>[2x]DYKDDDDKHHHHHHHHHHLEVLFQGPQSSERRVVAHMPGDIIIGALFSVHHQPTVDKVHERKCGAVREQYGIQRVEAMLHTLERINSDPTLLPNITLGCEIRDSCWHSAVALEQSIEFIRDSLISSEEEEGLVRCVDGSSSSFRSKKPIVGVIGPGSSSVAIQVQNLLQLFNIPQIAYSATSMDLSDKTLFKYFMRVVPSDAQQ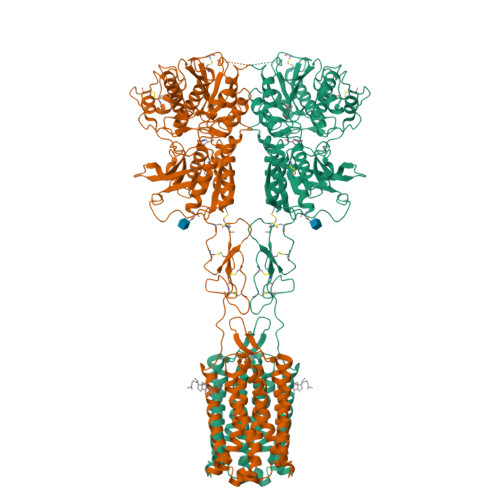ARAMVDIVKRYNWTYVSAVHTEGNYGESGMEAFKDMSAKEGICIAHSYKIYSNAGEQSFDKLLKKLTSHLPKARVVACFCEGMTVRGLLMAMRRLGLAGEFLLLGSDGWADRYDVTDGYQREAVGGITIKLQSPDVKWFDDYYLKLRPETNLRNPWFQEFWQHRFQCRLEGFPQENSKYNKTCNSSLTLKTHHVQDSKMGFVINAIYSMAYGLHNMQMSLCPGYAGLCDAMKPIDGRKLLESLMKTAFTGVSGDTILFDENGDSPGRYEIMNFKEMGKDYFDYINVGSWDNGELKMDDDEVWSKKSNIIRSVCSEPCEKGQIKVIRKGEVSCCWTCTPCKENEYVFDEYTCKACQLGSWPTDDLTGCDLIPVQYLRWGDPEPIAAVVFACLGLLATLFVTVVFIIYRDTPVVKSSSRELCYIILAGICLGYLCTFCLIAKPKQIYCYLQRIGIGLSPAMSYSALVTKTNRIARILAGSKKKICTKKPRFMSACAQLVIAFILICIQLGIIVALFIMEPPDIMHDYPSIREVYLICNTTNLGVVAPLGYNGLLILACTFYAFKTRNVPANFNEAKYIAFAMYTTCIIWLAFVPIYFGSNYKAITMCFSVSLSATVLLGCMFVPKVYIILAKPERNVRSAFTTSTVVRMHVGDGKSSSAA> EFKLSEGQRAIYNFHKKVRKDVKNCRIPGQPPAKNLTKLKWNKLLANKAKQQAKRCKYDSNDPNDF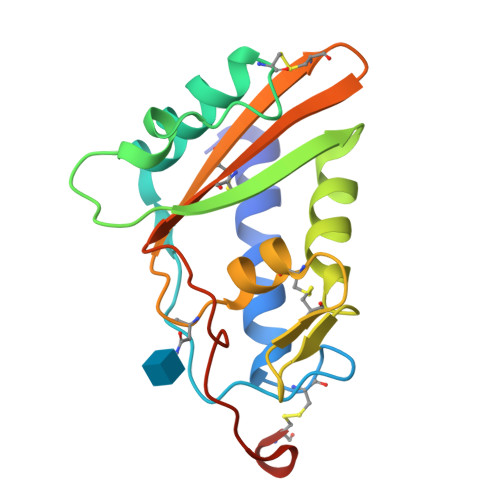IIGDFESIGQNLADYPTIEGAMKDWLEEYKNYNFEKNQCNGDCKNYKQMVWNTTEEIGCGYEKCGKNYLIVCNYAPGDSEDRPYEAKPESKCNKSE> DEAREAAAVRALVARLLGPGPAADFSVSVERALAAKPGLDTYSLGGGGAARVRVRGSTGVAAAAGLHRYLRDFCGCHVAWSGSQLRLPRPLPAVPGELTEATPNRYRYYQNVCTQSYSFVWWDWARWEREIDWMALNGINLALAWSGQEAIWQRVYLALGLTQAEINEFFTGPAFLAWGRMGNLHTWDGPLPPSWHIKQLYLQHRVLDQMRSFGMTPVLPAFAGHVPEAVTRVFPQVNVTKMGSWGHFNCSYSCSFLLAPEDPIFPIIGSLFLRELIKEFGTDHIYGADTFNEMQPPSSEPSYLAAATTAVYEAMTAVDTEAVWLLQGWLFQHQPQFWGPAQIRAVLGAVPRGRLLVLDLFAESQPVYTRTASFQGQPFIWCMLHNFGGNHGLFGALEAVNGGPEAARLFPNSTMVGTGMAPEGISQNEVVYSLMAELGWRKDPVPDLAAWVTSFAARR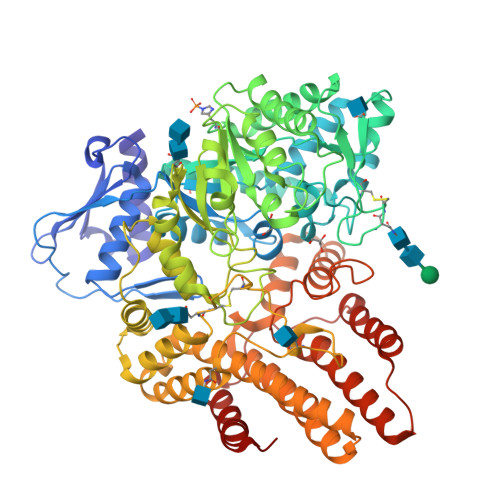YGVSHPDAGAAWRLLLRSVYNCSGEACRGHNRSPLVRRPSLQMNTSIWYNRSDVFEAWRLLLTSAPSLATSPAFRYDLLDLTRQAVQELVSLYYEEARSAYLSKELASLLRAGGVLAYELLPALDEVLASDSRFLLGSWLEQARAAAVSEAEADFYEQNSRYQLTLWGPEGNILDYANKQLAGLVANYYTPRWRLFLEALVDSVAQGIPFQQHQFDKNVFQLEQAFVLSKQRYPSQPRGDTVDLAKKIFLKYYPRWVAGSW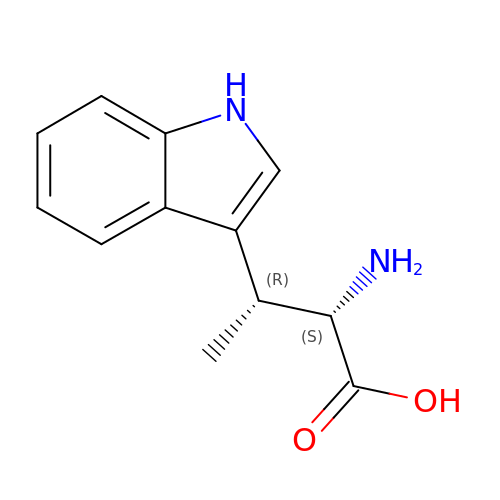(2S,3R)-2-azanyl-3-(1H-indol-3-yl)butanoic acid | C12 H14 N2 O2 | CZSQAYAIWDEOSA-HQJQHLMTSA-N undecan-2-one | C11 H22 O | 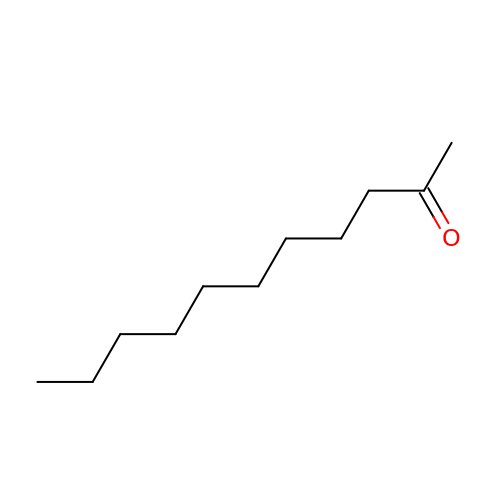KYWIYKKSMDLRDC-UHFFFAOYSA-N> MTLQQQIIKALGAKPQINAEEEIRRSVDFLKSYLQTYPFIKSLVLGISGGQDSTLAGKLCQMAINELRLETGNESLQFIAVRLPYGVQADEQDCQDAIAFIQPDRVLTVNIKGAVLASEQALREAGIELSDFVRGNEKARERMKAQYSIAGMTSGVVVGTDHAAEAITGFFTKYGDGGTDINPLYRLNKRQGKQLLAALACPEHLYKKAPTADLEDDRPSLPDEVALGVTYDNIDDYLEGKNVPQQVARTIEN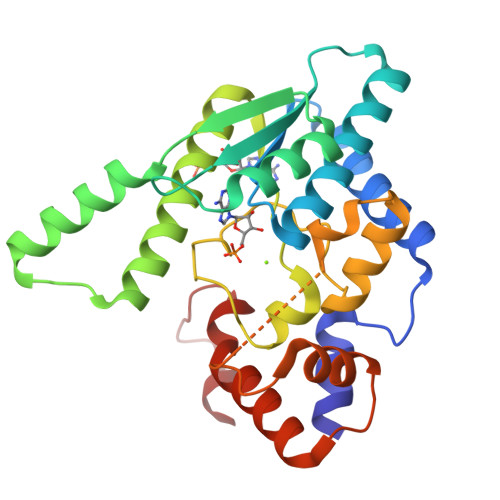WYLKTEHKRRPPITVFDDFWKK> GSEAWFNEKSKELTTEIDNNIEQISSYKSEITELRRNVQAL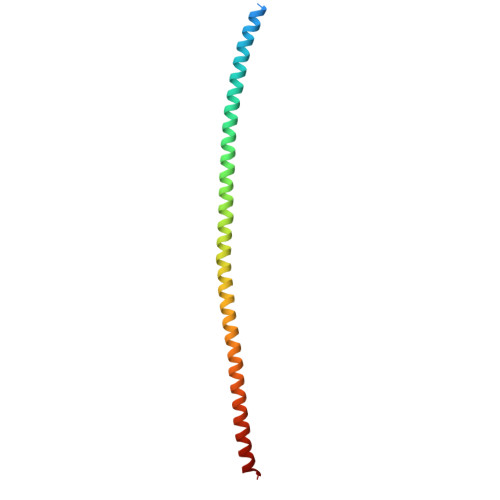EIELQSQLALKQSLEASLAETEGRYAVQLSQIQAQISALEEQLQQIRAETECQNTEYQQLLDIKIRLENEIQTYRSLLEGE>[2x]MTQERKVALVTGASRGIGAAIAQQLIQDGYFVVGTATS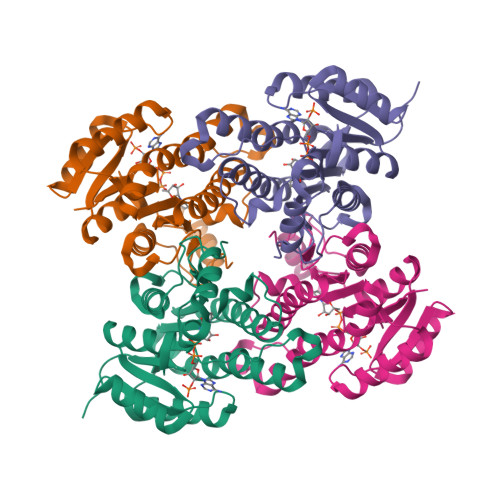ESGAQKLTDSFGEQGAGLALDVRNLDEIEAVVSHIEQNYGPVLVLVNNAGITKDNLLLRMSEDDWDDILNIHLKAVYRLSKRVLKGMTKARFGRIINISSVVAHFANPGQANYSAAKAGIEAFSRSLAKEMGSRQITVNSVAPGFIATEMTDALSEDIRKKMSDQVALNRLGEPQDIANAVSFLASDKAGYITGTVLHVNGGLYMA>[2x]CGLVASNLNLKPGECLRVRGEVAPDAKSFVLNLGKDSNNLCLHFNPRFNAHGDANTIVCNSKDGGAWGTEQREAVFPFQPGSVAEVCITFDQANLTVKLPDGYEFKF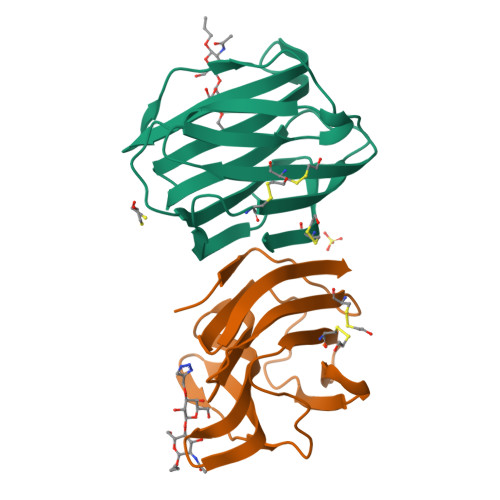PNRLNLEAINYMAADGDFKIKCVAFD ZER1 and ZYG11B, the substrate receptors of the Cullin 2-RING E3 ubiquitin ligase (CRL2), recognize N-terminal (Nt) glycine degrons and participate in the Nt-myristoylation quality control through the Gly/N-degron pathway. Here we show that ZER1 and ZYG11B can also recognize small Nt-residues other than glycine. Furthermore, we present the crystal structures of ZER1 and ZYG11B bound to various small Nt-residues and uncover the molecular mechanism of non-acetylated substrate recognition by ZER1 and ZYG11B. In conclusion, we propose that ZER1/ZYG11B not only targets Gly/N-degrons for proteasomal degradation, but it also has the ability to bind a defined selection of non-Ac/N-degrons by a conserved molecular mechanism of substrate recognition and target their degradation through the non-Ac/N-degron pathway.

To understand the molecular basis of ZER1/ZYG11B-mediated binding of non-Gly Nt-residue peptides, we determined the crystal structures of ZER1 bound to either SFLH-, AFLH- or TFLH-peptide, as well as the crystal structures of ZYG11B bound to either SFLH-, AFLH- or CFLH- peptide. In line with our SPOT-array results, ZER1 binds to XFLHVGQD peptides in which X is either Ser (KD of 1.3), Ala (KD of 1.6), Thr (KD of 3.1) or Cys (KD of 3.9) more potently than to the Gly-starting peptide (KD of 4.2). Structural comparisons indicated that the peptide-binding modes of ZER1 and ZYG11B are similar. In this cavity, the main chains of the first three residues of the bound peptides are coordinated by a set of conserved hydrogen bonds. The free α-amino group of the Nt-residue forms hydrogen bonds with the side chains of Asp556 and Asn597 in ZER1 (the counterparts of Asp 526 and Asn 567 in ZYG11B), respectively. Furthermore, the carbonyl oxygen of the Nt-residue is stabilized by two hydrogen bonds from Asn597 and Trp552 in ZER1 (Asp 567 and Trp522 in ZYG11B). The main-chain amide and carbonyl of the second residue (F2) on the peptide hydrogen bond to the main-chain respective carbonyl and amide of Asn679 in ZER1 (Ala647 in ZYG11B). Besides, a strong π-π interaction was formed between the aromatic side chain of F2 and the indole ring of Trp 552 in ZER1 (Trp 522 in ZYG11B), this observation is consistent with our SPOT-array results that ZER1 and ZYG11B prefer an aromatic residue at position 2. The main-chain amide of the third residue on the peptide is anchored by a hydrogen bond with Asn553 in ZER1 (Asn523 in ZYG11B). Our ITC assays indicated that any alanine mutation of W552, D556, N597 or E600 in ZER1, which would disrupt the direct hydrogen bonds with Nt-residue, abolished the binding to the XFLHVGQD (X = Ser, Ala, Cys or Thr) peptides, highlighting the key role of these hydrogen bonds in mediating Nt-residue recognition.

>[4x]AFLHVGKMGFVVTMLKLIQKKLLDKTCDQVMEFSWSALWNITDETPDNCEMFLNFNGMKLFLDCLKEFPEKQELHRNMLGLLGNVAEVKELRPQLMTSQFISVFSNLLESKADGIEVSYNACGVLSHIMFDGPEAWGVCEPQREEVEERMWAAIQSWDINSRRNINYRSFEPILRLLPQGISPVSQHWATWALYNLVSVYPDKYCPLLIKEGGMPLLRDIIKMATARQETKEMARKVIEHCSNFKEENMDTSR>[2x]KTPLVNESLKKFLNTKDGRLVASLVAEFLQFFNLDFTLA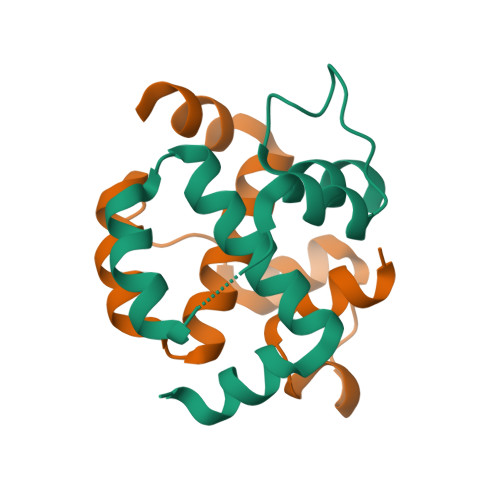VFQPETSTLQGLEGRENLARDLGIIEAEGTVGGPLLLEVIRRW1-methyl-3-[3-(2-methylpyrimidin-4-yl)phenyl]urea | C13 H14 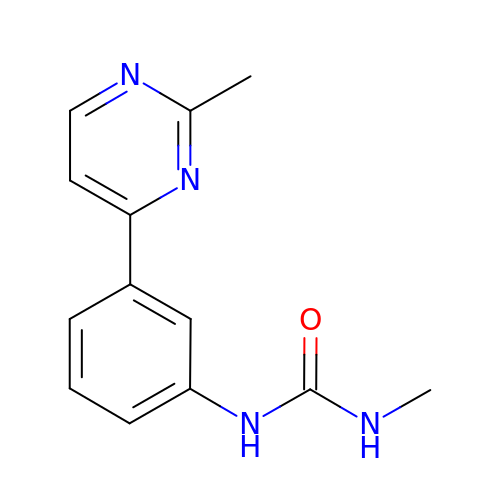N4 O | AEADJOBCASCCHA-UHFFFAOYSA-N N-[2-(cyclohex-1-en-1-yl)ethyl]-3,5-dimethyl-1,2-oxazole-4-carboxamide | C14 H20 N2 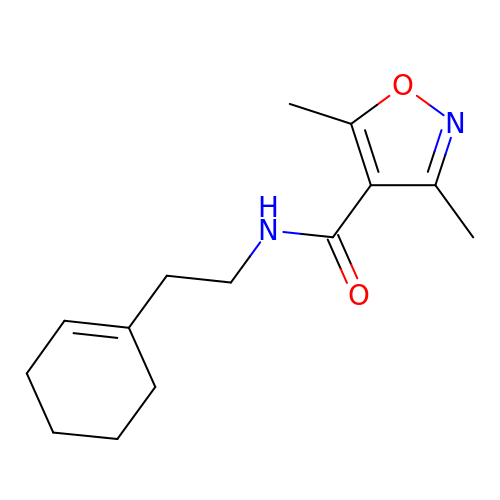O2 | CDMDKICUIFSGRO-UHFFFAOYSA-N[[(2R,3S,4R,5R)-5-(4-azanyl-2-oxidanylidene-pyrimidin-1-yl)-3,4-bis(oxidanyl)oxolan-2-yl]methoxy-oxidanyl-phosphoryl]oxy-(2-hydroxyethyl)phosphinic 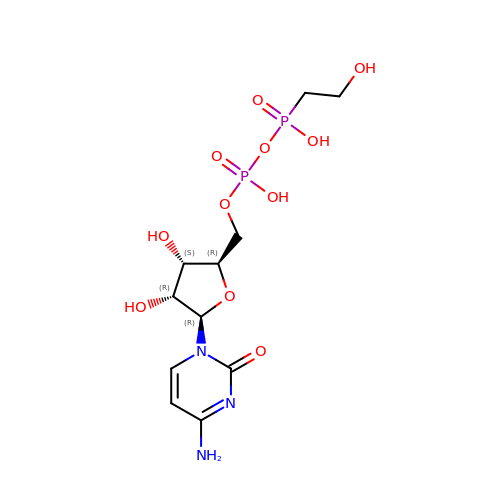acid | C11 H19 N3 O11 P2 | ODFOOQGQRDVSPW-PEBGCTIMSA-N> SVRYLGRVNPATKELSWPGTGVSFAFTGTSATIGIASVSGTNSVDLVIDGGEPIVISDFAGTGISTPAGLRKGKHTVVLRRRSEPAYGSIFLGNITTDGHFVPTAPAPKRQIDIIGDSITVGYGLDGTFPCTNTAALEDNPKTYGVLAANALGADYSVVAWSGKGLIRNFASGSPDTSPLMPQLYTRYGANDADGSYPFPRSWSPDAVVINLGTNDFGYLGVRDPIDVAAYTDAMVKFVQDIQKHYPRAHFFLLNSPMLSDTWPTAADAQK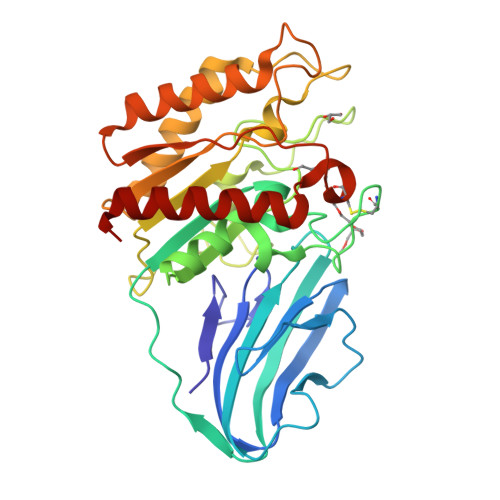TTQTNAIKNAVSRLGAKAHFVDWPTQGSDVGCDYHPNAATHAAEGEVLAKAIAAALGW>MKLQVLQVLDRLKMKLQEKGDTSQNEKLSMFYETLKSPLFNQILTLQQSIKQLKGQLNHILESGKETAAAKFERQHMDSSTSA[2x];>MGSSHHHHHHSQDPDVEDLFSSL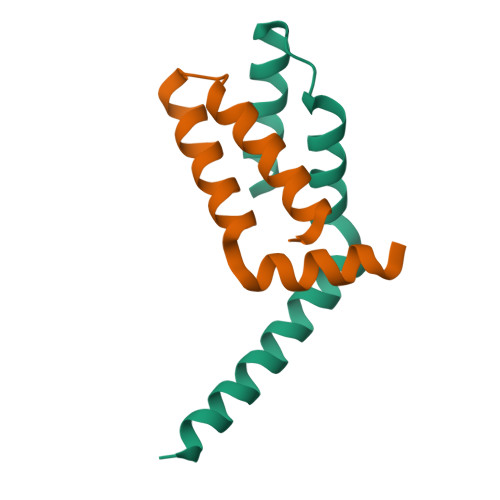KHIQHTLVDSQSQEDISLLLQLVQNRDFQNAFKIHNAVTVHMSKASPPF[2x]> LRPKLSEEQQRIIAILLDAHHKTYDPTYSDFCQFRPPVRVNDGGGSVTLELSQLSMLPHLADLVSYSIQKVIGFAKMIPGFRDLTSEDQIVLLKSSAIEVIMLRSNESFTMDDMSWTCGNQDYKYRVSDVTKAGHSLELIEPLIKFQVGLKKLNLHEEEHVLLMAICIVSP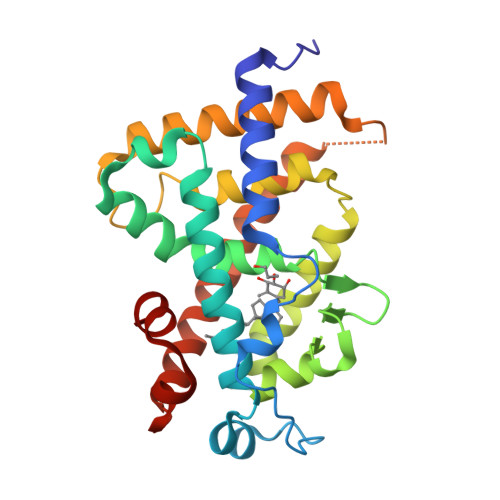DRPGVQDAALIEAIQDRLSNTLQTYIRCRHPPPGSHLLYAKMIQKLADLRSLNEEHSKQYRCLSFQPECSMKLTPLVLEVFG(2R)-1-(pyrrolidin-1-yl)-3-(9H-thioxanthen-9-yl)propan-2-ol | 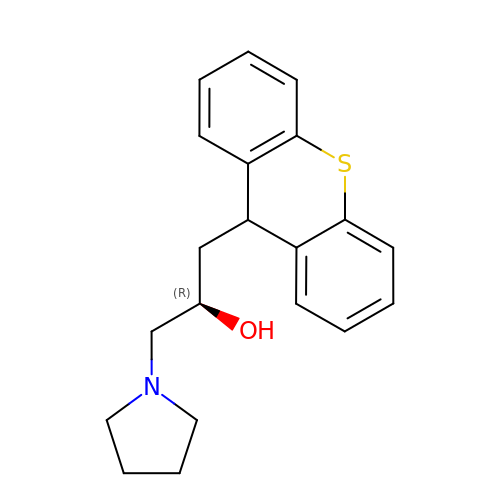C20 H23 N O S | SJCVUEZFZDNDKT-OAHLLOKOSA-N>[4x]RLFGTAGIRGTLWEKVTPELAMKVGMAVGTYKSGKALVGRDGRTSSVMLKNAMISGLLSTGMEVLDADLIPTPALAWGTRKLADAGVMITASHNPPTDNGVKVFNGDGTEFYVEQERGLEEIIFSGNFRKARWDEIKP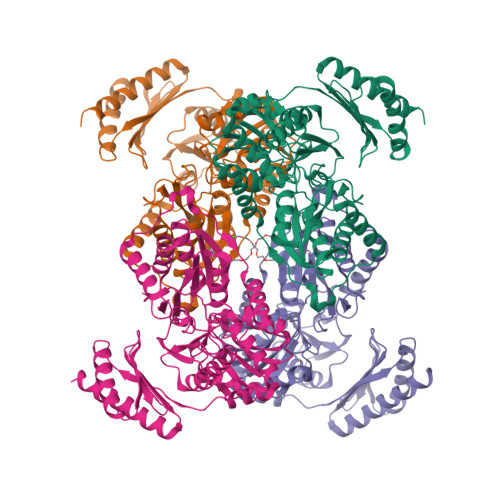VRNVEVIPDYINAVLDFVGHETNLKVLYDGANGAGSLVAPYLLREMGAKVLSVNAHVDGHFPGRKPEPRYENIAYLGKLVRELGVDLAIAQDGDADRIAVFDEKGNYVDEDTVIALFAKLYVEEHGGGTVVVSIDTGSRIDAVVERAGGRVVRIPLGQPHDGIKRYKAIFAAEPWKLVHPKFGPWIDPFVTMGLLIKLIDENGPLSELVKEIPTYYLKKANVLCPDEYKAEVVRRAAEEVERKLSSEIKEVLTISGFRIALNDGSWILIRPSGTEPKIRVVAEAPTEKRRDELFEMAYSTVSRIVKEAEKK>GMDKYREIHNKLKEFSPGTLTAVECIDYLD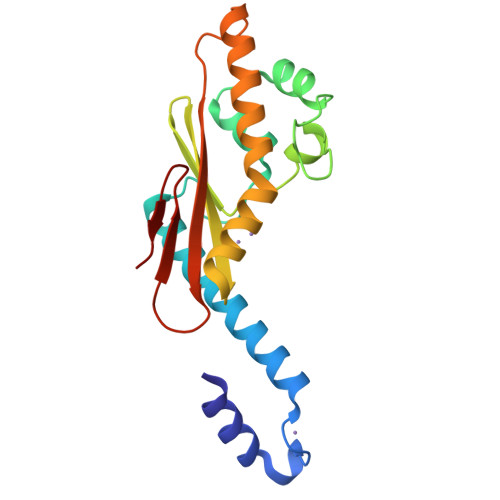RLYAVRHDIVDQMIKHDWSDNKDSEEAIGKVLLFAGVPSNIITALEKKIIPNHPTGKSLKAFFKMTPDNYKISGTTIEFVEVTVTADVDKGIREKKLKYEAGLTYIEQELHKFFLKGEIPQPYKITFNVVAVRTDGSNITTQWPSRRNDG[2x]> GPGSELPQMVQQLNSPDQQELQSALRKLSQIASGGNEQIQKLIEAGALSPLVKLLDDASEEVIKEAVWAIANIASGNNEQIQKLIEAGALSPLVKLLDDASEEVIKEAVWAIANIASGNNEQIQKLIEAGALSPLVKLLDDASEEVIKEAVWAIANIASGNNEQIQKLIEAGALSPLVKLLDDASEEVIKEAVWAIANIASGNNEMKQKLE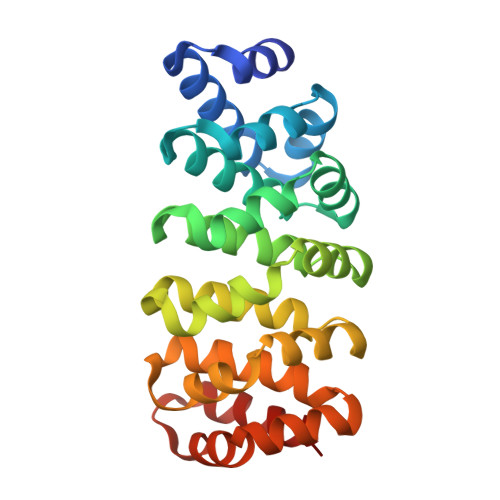EAGALPALEKLQSHANEEVQKNAQAALEAFNS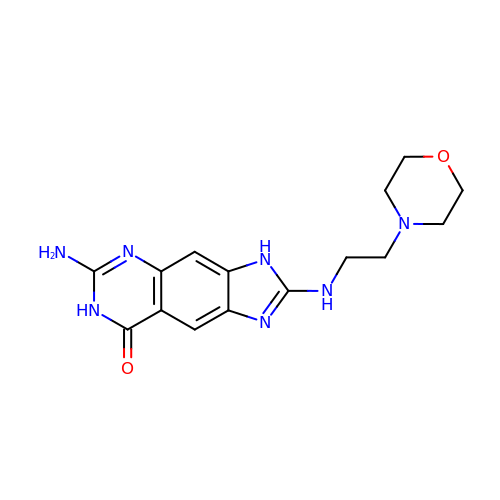6-amino-2-[(2-morpholin-4-ylethyl)amino]-3,7-dihydro-8H-imidazo[4,5-g]quinazolin-8-one | C15 H19 N7 O2 | JUHXOBNFTFUPKQ-UHFFFAOYSA-N>MGHHHHHHHHLVPRGSMFADLDYDIEEDKLGIPTVPGKVTLQKDAQNLIGISIGGGAQYCPCLYIVQVFDNTPAALDGTVAAGDEITGVNGRSIKGKTKVEVAKMIQEVKGEVTIHYNKLQQSAV[2x]

Protein interacting with kinase C1 (PICK1) is a membrane protein composed of a N‐terminal PDZ domain and a C‐terminal BAR domain, and is expressed highly in the brain and peripheral tissues. It functions as an intracellular trafficking protein involved in the internalization of amino‐3‐hydroxyl‐5‐methyl‐4‐isoxazole‐propionate (AMPA) type receptors which are localized on the surface of neurons and mediate synaptic communication. The PDZ domain of PICK1 recognizes and binds to the intracellular PDZ binding motif on the c‐terminus of GluA2. PICK1's PDZ domain is unique in its ability to bind both class I and II motifs, however, it binds class II motifs (i.e., GluA2 (SVKI)) with a 10‐fold‐higher affinity over class I motifs (i.e., PKCα (QSAV)).

We fused the class 1 PDZ binding motif QSAV from PKCα to the C‐termini of the PICK1 PDZ domain to enhance solubility and aid crystallization. The purified PICK1 PDZ‐QSAV protein eluted as a dimer on size exclusion chromatography under reducing conditions indicating that we successfully designed an intramolecular interaction between the PDZ domains using the fused QSAV extension. The structure revealed electron density that confirmed that the dimer was locked by two disulfide bounds between C44(A)‐C46(B) and C44(B)‐C46(A) between the two PDZ domain chains of PICK1. However, because electron density for the fused QSAV tail from the dimeric partner peptide was visible in the peptide groove, this method failed in allowing BIO124 to displace the QSAV tail within the crystal lattice. The crystal structure that was obtained in the attempt to co‐crystallize with BIO124 represents the first PICK1 structure bound to a class I PDZ binding motif (QSAV from PKCα). The class 1 PKCα QSAV peptide has an alanine at the −1 position and is unable to make this interaction. The second difference is between the polar and nonpolar sidechains at the −2 position. The polar serine of the class I QSAV does not make an interaction to K83 in the αB1 position in PICK1. In the class II SVKI, the hydrophobic valine sidechain at −2 position forms a lipophilic interaction with the aliphatic segment of the Lys83 sidechain in the S–2 subpocket. These two additional lipophilic interactions support the observations that class II peptides demonstrate higher binding affinities for PICK1 over class I peptides.>[12x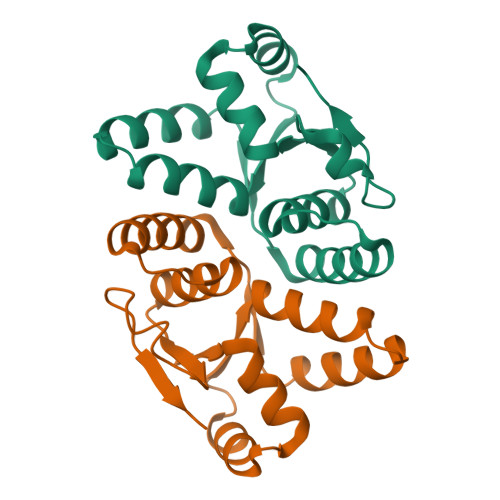]MHHHHHHLKFMLNTNICIFTIKNKPASVRERFNLNQGKMCISSVTLMELIYGAEKSQMPERNLAVIEGFVSRIDVLDYDAAAATHTGQIRAELARQGRPVGPFDQMIAGHARSRGLIIVTNNTREFERVGGLRTEDWS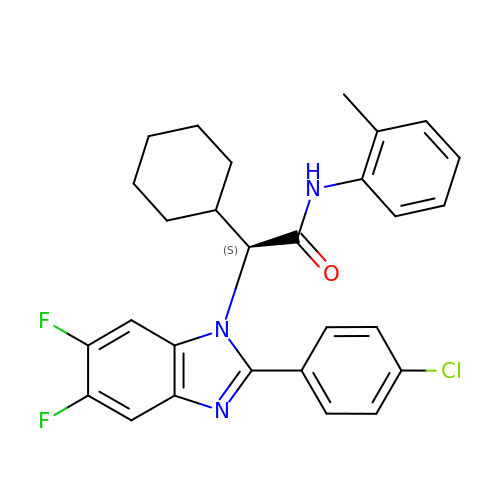(2S)-2-[2-(4-chlorophenyl)-5,6-difluoro-1H-benzimidazol-1-yl]-2-cyclohexyl-N-(2-methylphenyl)ethanamide | C28 H26 Cl F2 N3 O | LUMVOGPLODDMEP-SANMLTNESA-N>MAFCFGSFFSKYASSKSGSQARYRFLHSSAKIAAGATGALLLGGATVALCYFPSGRKVTEAPPFDVNSLRRDIEEILSEDMSKGPLFVRLAWHEAGSWDCRKKDGSPNSASMRFHPECSYAGNKGLDKGRNALESLKKKYPKISYADLWSFAAVVSIEAMGGPEIPWRWGRVDAKDGSVCGPDGRLPDASRMQDHVRDVFSRLGFNDEETVALIGAHTCGECHLENTGYVGPWTHDKYGFDNSFFTELFGNEWMLNPNVKKMQFMDKTTNRLMMLPADVSILLDDKYRSIAKKYADDNDYFCNAFSKAYQKLLEVGTTDLKSLPAESK[2x]

One of these is a hybrid heme peroxidase, the T. cruzi ascorbate peroxidase-cytochrome c peroxidase enzyme (TcAPx-CcP). TcAPx-CcP has high sequence identity to members of the class I peroxidase family, notably ascorbate peroxidase (APX) and cytochrome c peroxidase (CcP), as well as a mitochondrial peroxidase from Leishmania major (LmP). Like LmP, TcAPx was later found to have both ascorbate and cytochrome c activity and was thus renamed as TcAPx-CcP. Integration of steady state kinetic experiments, molecular dynamic simulations, and bioinformatic analyses indicates that TcAPx-CcP preferentially oxidizes cytochrome c but is still competent for oxidization of ascorbate.

The TcAPx-CcP enzyme is similar in its overall structure to the related LmP enzyme with which TcAPx-CcP shares 57% sequence identity. The structure comprises of 10 α-helical bundles, which is consistent with the characteristics of other peroxidase structures. TcAPx-CcP also features a limited amount of ordered β-structure (located approximately between Gly250-Asn270), which has until now only been identified in CcP and to a slightly lesser extent LmP. The active site of TcAPx-CcP comprises Trp92 in the distal pocket, along with distal histidine (His93) and arginine (Arg89) residues. On the proximal side there is a typical peroxidase His217-Asp278-Trp233 proximal triad, as observed in yeast CcP and in soybean APX (sAPX, His163-Asp208-Trp179). There are two molecules in the asymmetric unit for both the wild type and mutant structures, each one exhibiting different electron density at the distal heme position, with one appearing to bind an oxygen molecule and another a water molecule approximately 2.3 Å above the iron (not shown). No equivalent Arg residue is present in TcAPx-CcP, and this residue is instead replaced with Asn226, which is fully conserved in every T. cruzi genome evaluated.>GMPLLIDIRKLTLITRLIQDGAEQVADSLATLAGVDAAVEIKSLSFVQPEDIATEMGGGTIYSARVRLTEPPYGVFLMTFETETAAEIAELMTGSSVEDGFTQLHESALQEMCNILTSGFIDGIANTLNATINMGTPTVVQDDATEIADKA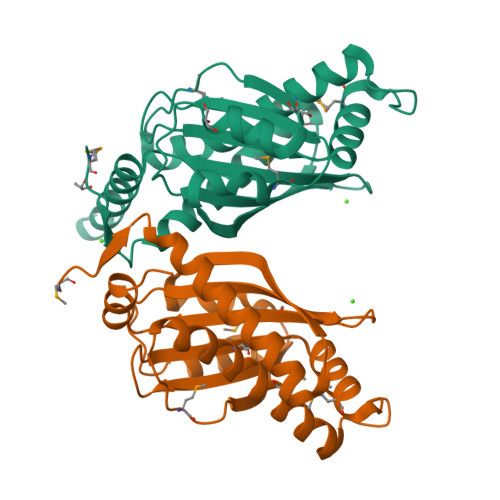LSHVRRDSLTIVLDSLVDIKESDVAFSLRIFLIPDPGSFVHLIDQLDYDTDRETHISADTDAVKELDMSGDADALDAFDSSK[2x]> GPEIVDTCSLASPASVCRTKHLHLRCSVDFTRRTLTGTAALTVQSQEDNLRSLVLDTKDLTIEKVVINGQEVKYALGERQSYKGSPMEISLPIALSKNQEIVIEISFETSPKSSALQWLTPEQTSGKEHPYLFSQCQAIHCRAILPCQDTPSVKLTYTAEVSVPKELVALMSAIRDGETPDPEDPSRKIYKFIQKVPIPCYLIALVVGALESRQIGPRTLVWSEKEQVEKSAYEFSETESMLKIAEDLGGPYVWGQYDLLVLPPSFPYGGMENPCLTFVTPTLLAGDKSLSNVIAHQISHSWTGNLVTNKTWDHFWLNEGHTVYLERHICGRLFGEKFRHFNALGGWGELQNSVKTFGETHPFTKLVVDLTDIDPDVAYSSVPYEKGFALLFYLEQLLGGPEIFLGFLKAYVEKFSYKSITTDDWKDFLYSYFKDKVDVLNQVDWNAWLYSPGLPPIKPNYDMTLTNACIALSQRWITAKEDDLNSFNATDLKDLSSHQLNEFLAQTLQRAPLPLGHIKRMQEVYNFNAINNSEIRFRWLRLCIQSKWEDAIPLALKMATEQGRMKFTRPLFKDLAAFDKSHDQAVRTYQEHKASMHPVTAMLVGKDLKVD;> PGP

LTA4H catalyzes the final and rate limiting step in the biosynthesis of pro-inflammatory LTB4, that is, the vinylogous hydrolysis of the epoxide, LTA4. LTA4 binds to a deep L-shaped hydrophobic channel which forms one of two lobes of the catalytic site of the enzyme. The second lobe of the catalytic site of LTA4H is a more open and hydrophilic pocket, and forms the aminopeptidase activity of the enzyme. While less is known about the physiological relevance of the aminopeptidase activity of LTA4H, Snelgrove and co-workers suggested that it can degrade the tripeptide PGP which has been reported to be a collagen-derived matrikine and neutrophil chemoattractant.

Overlaying the structure of LTA4H bound JNJ-26993135 (compound 11) to that of PGP bound in the active site showed that simultaneous binding of the two ligands would not be possible due to steric effects. However, we hypothesized that by removing the part of the compound which interacts with the Zn2+, we would be able to have simultaneous binding of the PGP and the truncated compound to LTA4H. On the other hand, in the exudate of the LTA4H KO mice, over 80% of the PGP was still present even after 24 h, suggesting that LTA4H is the dominant enzyme for degradation of PGP in vivo. In both exudates, Ac-PGP remained as stable over 24 h at 37 °C as in PBS. This indicated that, as already observed by others, LTA4H cannot degrade the acetylated version of PGP. Although LTA4H is the dominant enzyme that can degrade PGP in vivo, the physiological relevance of this activity seems highly questionable.>MVSTTETAAAGPAKTSKKQDEGLVTNKYKPKEPYVGRCLS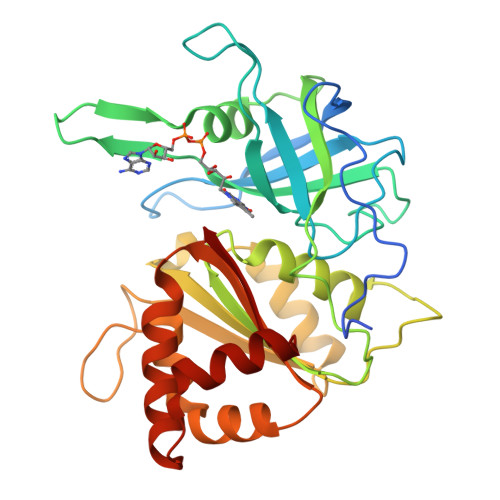NTRITGDDAPGETWHMVFSTEGEIPYREGQSIGIIADGEDKNGKPHKLRLYSIASSALGDFGDSKTVSLCVKRLVYTNDQGEIVKGVCSNFLCDLKPGADVKITGPVGKEMLMPKDPNATVIMLATGTGIAPFRSFLWKMFLEEHEDYKFSGLAWLFLGVPTSDSLLYKEELEKMKEMAPDNFRLDFAVSREQTNAAGEKMYIQTRMAEYREELWELLKKDNTYVYMCGLKGMEKGIDDIMLNLAAKDGIDWMQYKKQLKKGEQWNVEVY[2x]Prenyltransferases, also known as isoprenyl diphosphate synthases, catalyze the sequential condensation of a basic five-carbon building block (C5), the isopentenyl diphosphate (IPP), to synthesize prenyl precursors of isoprenoid metabolites and isoprene polymers, collectively called polyisoprene. Ultrahigh molecular weight cis-1,4-polyisoprene and trans-1,4-polyisoprene (TPI), which are the principal components of natural rubber and gutta-percha, respectively, are also isoprenoid metabolites that are assumed to be synthesized by specialized prenyltransferases. These prenyltransferases are divided into two major groups, the cis-1,4-prenyltransferases (CPTs) and trans-1,4-prenyltransferases (TPTs), based on the stereochemistry of the double bond formed during IPP condensation. To investigate the molecular properties of the EuTPT proteins, we determined the three-dimensional structures of EuTPT3 and EuFPS1 using X-ray crystallography. Similar to EuFPS1 and other prenyltransferases, the EuTPT3 subunits were composed of 10 core helices (α1-α10) with a deep pocket that included two DDxxD motifs responsible for substrates binding.

The crystal structure of apo EuTPT3 was determined from two crystal forms with space groups P43212 and C2, refined at 3.0 and 3.3 Å resolution, respectively. All dimers observed in the two crystal forms were superimposable with a root-mean-square deviation (RMSD) range of 0.797–0.941 Å over 595–633 aligned Cα atoms. The superimposition parameters suggested that the dimeric architecture of EuTPS3 was highly conserved and unlikely to be caused by crystal packing. In EuTPT3, α6 of one subunit interacted with α5 and α6 of the neighboring subunit to form a four-helix bundle, whereas, in EuFPS1, α4 of one subunit was inserted between α5 and α6 of the neighboring subunit to form a six-helix bundle of α4–α6 at the dimer interface. Thus, EuTPT3 had a larger central tunnel than EuFPS1. The tunnel is mainly composed by hydrophobic residues of α5 and α6, which is considered the path for the products because the chain length determination element locates in this region. Among the structural elements involved in substrate binding and catalytic activity, EuTPT3 featured two conserved DDxxD motifs at the active site, both of which could contribute to substrate recognition. EuTPT3 also featured structurally conserved basic residues (Lys46, Arg50, Arg109, and Lys348) in the equivalent positions. Crystal structure of EuTPT3 showed that the residues Ile164-Ala165 contact with Ile164 and Ile125 of the neighboring subunit in the hydrophobic tunnel, suggesting that smaller side chains such as valine and glycine provide the wider path for the product that may contribute to the activity difference.

>MNHKVHHHHHHIEGRHMTELKSKFVKVYSVLKKELLHDSAFGLTDDSRNWVERIMDYNVPGGKLNRGLSVVDSYKLLRELTNSKYKSELSDDEIFLASVLGWSVEWIQACALVLDDIMDHSHTRRGHPCWFRLPKVGMIAINDGLILRNHVPRILRTHFQTEHYYLQLVDLFHEVECQTIAGQMLDLITTLAGEINLSSYSLPVYQQITLSKTSYYSFYLPVACALVMLGENLESHDDMKDILLEMGTYFQVQDDYLDCFGDPEVIGKIGTDIEDNKCTWLVVQALEHCNEEQKKLLYDNYGRKDPKQVAKVKELYKTLNLEDLFTQYENKTCKKLTKSIEALPNVAVQAVLKSFLAKIHKRLK[2x]> SPRPFNEIPSPGDNGWLNLYHFWRETGTHKVHLHHVQNFQKYGPIYREKLGNVESVYVIDPEDVALLFKSEGPNPERFLIPPWVAYHQYYQRPIGVLLKKSAAWKKDRVALNQEVMAPEATKNFLPLLDAVSRDFVSVLHRRIKKAGSGNYSGDISDDLFRFAFESITNVIFGERQGMLEEVVNPEAQRFIDAIYQMFHTSVPMLNLPPDLFRLFRTKTWKDHVAAWDVIFSKADIYTQNFYWELRQKGSVHHDYRGILYRLLGDSKMSFEDIKANVTEMLAGGVDTTSMTLQWHLYEMARNLKVQDMLRAEVLAARHQAQGDMATMLQLVPLLKASIKETLRLHPISVTLQRYLVN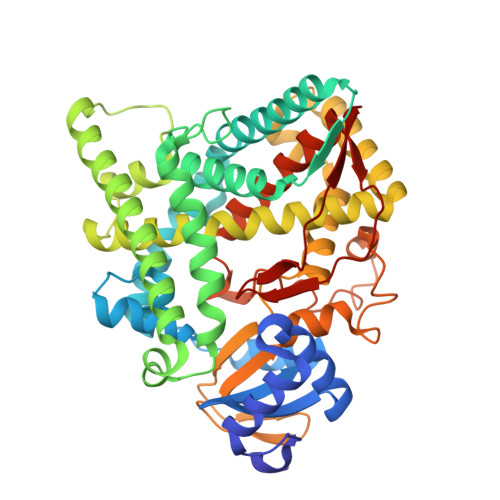DLVLRDYMIPAKTLVQVAIYALGREPTFFFDPENFDPTRWLSKDKNITYFRNLGFGWGVRQCLGRRIAELEMTIFLINMLENFRVEIQHLSDVGTTFNLILMPEKPISFTFWPF>GANAMAHMIGVYITKWGFEVETFKKALPKNTEVKTIAFTGDWIEAVRQFYSTVKEIDGHIHLALNGPSSLAFGCGVIFGSLKTFSFWHYQNGAYHTIPITNVRALKQRLKQYNYVEPFYEAGGKDLVVMLNYSHHEIKTAVKEYVMNKLRLENPSYLEISLKGITGNIPIELMPTVANETSSLLQDVKKHQSFDRFHFFFSCPVPIAFMVGVAFGLYDELVVYNFSGTYEPVLSFKDLK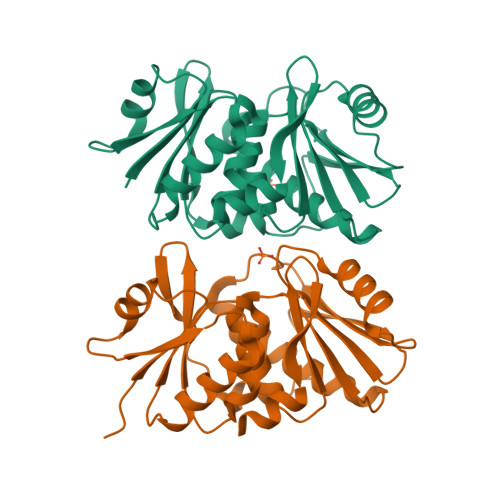EVKL[2x]>SNAMTAPRAWRPIAGGPPAGPLVLAVDFAATGRPEAAFADLVARLDPGTEVWESLQPPLGTETGMVAEDYVTRWEEEVRASGRRIGAVLGFSAGSAFAGELAVRLARSQPRSPRLVVFDPESPTTSTLYYQFRKVVESLAGVLGEQAAREALAEGTAAADRIGDVEGLGAELVRVFTAAGRAACAAADLDDEFADELTATYRSFVSYLVAAAAVDHVKCWSGAVAVSSATPTSGLNPLDPAARAALVERELTFDVHHADLLRDPGVARAVARLLA[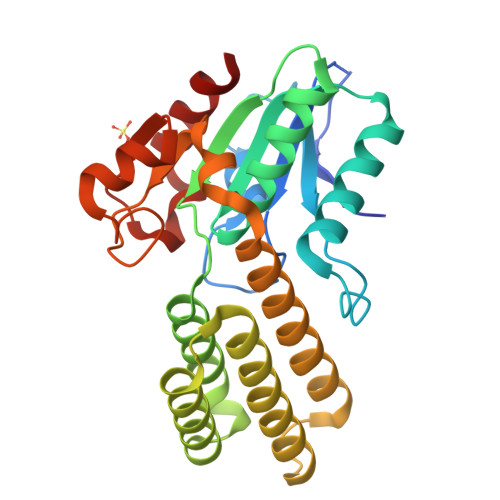2x]> SMSGRVGDLSPKQAETLAKFRENVQDVLPALPNPDDYFLLRWLRARNFDLQKSEALLRKYMEFRKTMDIDHILDWQPPEVIQKYMPGGLCGYDRDGCPVWYDIIGPLDPKGLLFSVTKQDLLKTKMRDCERILHECDLQTERLGKKIETIVMIFDCEGLGLKHFWKPLVEVYQEFFGLLEENYPETLKFMLIVKATKLFPVGYNLMKPFLSEDTRRKIIVLGNNWKEGLLKLISPEELPAQFGGTLTDPDGNPKCLTKINYGGEIPKSMYVRDQVKTQYEHSVQINRGSSHQVEYEIL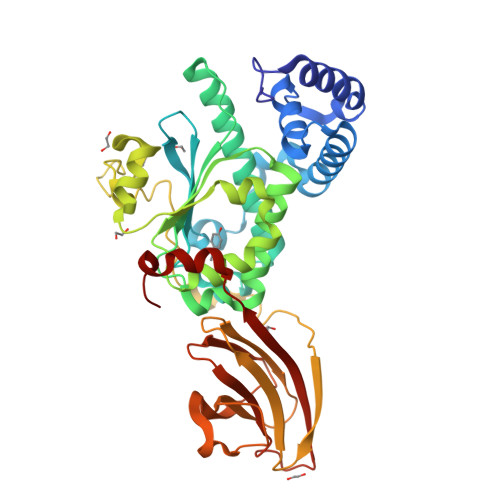FPGCVLRWQFSSDGADIGFGVFLKTKMGERQRAGEMTEVLPSQRYNAHMVPEDGNLTCSEAGVYVLRFDNTYSFVHAKKVSFTVEVLLPDEGMQKYDKELTPV4-(dimethylamino)-N-[5-(1H-indol-4-yl)pyridin-3-yl]butanamide 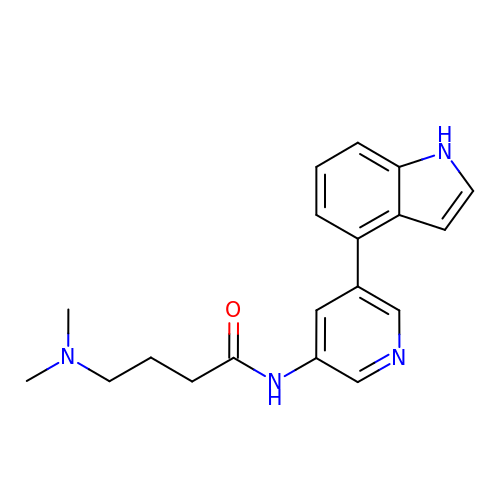| C19 H22 N4 O | QVBOWRMZONBBIK-UHFFFAOYSA-N1-(5-TERT-BUTYL-1,2-OXAZOL-3-YL)-3-(4-PYRIDIN-4-YLOXYPHENYL)UREA | C19 H20 N4 O3 | 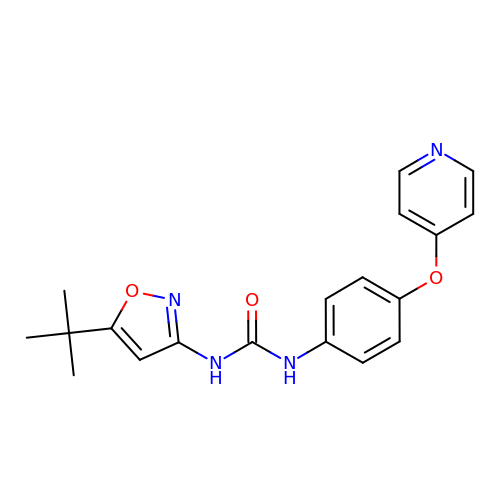XKNAGLMNQADBQE-UHFFFAOYSA-N> RAPPQFVVRPRDQIVAQGRTVTFPCETKG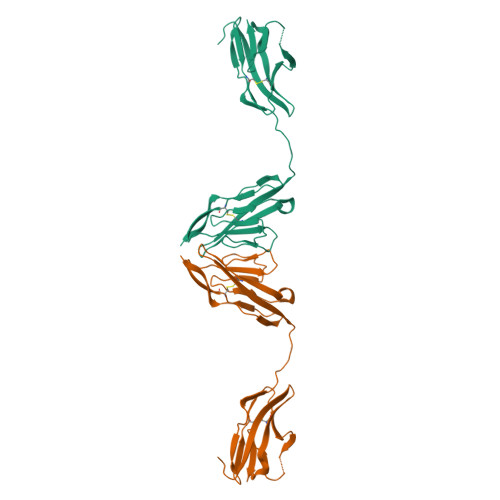NPQPAVFWQKEGSQNLLFPNQPQQPNSRCSVSPTGDLTITNIQRSDAGYYICQALTVAGSILAKAQLEVTDVLTDRPPPIILQGPAMQTLAVDGTALLKCKATGDPLPVISWLKEGFTFPGRDPRATIQEQGTLQIKNLRISDTGTYTCVATSSSGETSWSAVLDVTESGKL>[2x]GPGGDPHMGLNDNKAGMEGLDKEKINKIIMEATKGSRFYGNELKKEKQVNQRIENMMQQKAQITSQQLRKAQLQVDRFAMELEQSRNLSNTIVHIDMDAFYAAVEMRDNPELKDKPIAVGSMSMLSTSNYHARRFGVRAAMPGFIAKRLCPQLIIVPP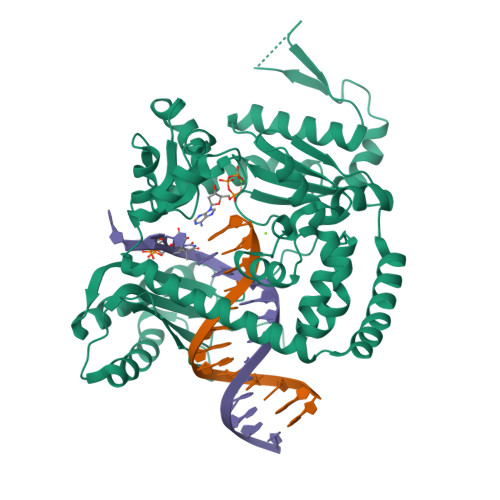NFDKYRAVSKEVKEILADYDPNFMAMSLDEAYLNITKHLEERQNWPEDKRRYFIKMGSSVENDNPGKEVNKLSEHERSISPLLFEESPSDVQPPGDPFQVNFEEQNNPQILQNSVVFGTSAQEVVKEIRFRIEQKTTLTASAGIAPNTMLAKVCSDKNKPNGQYQILPNRQAVMDFIKDLPIRKVSGIGKVTEKMLKALGIITCTELYQQRALLSLLFSETSWHYFLHISLGLGSTHLTRDGERKSMSVERTFSEINKAEEQYSLCQELCSELAQDLQKERLKGRTVTIKLKNVNFEVKTRASTVSSVVSTAEEIFAIAKELLKTEIDADFPHPLRLRLMGVRISSFPNEEDRKHQQRS> MAKDIEISASESKFILEALRQNYRLDGRSFDQFRDVEITFGKEFGDVSVKMGNTKVHCRISCQIAQPYEDRPFEGLFVISTEISPMAGSQFENGNITGEDEVLCSRIIEKSVRRSGALDVEGLCIVAGSKCWAVRADVHFLDCDGGFIDASCIAVMAGLMHFKKPDITVHGEQIIVHPVNEREPVPLGILHIPICVTFSFFNPQDTEENIKGETNSEISIIDATLKEELLRDGVLTVTLNKNREVVQVSKAGGLPMDALTLMKCCHEAYSIIEKITD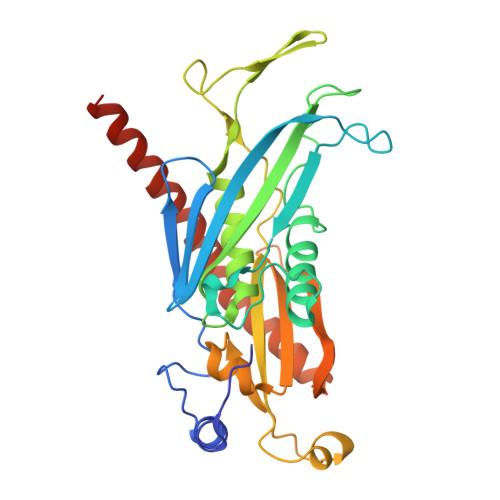QILQLLKEDSEKRNKYAAMLTSENAREI>[2x]MDAQYDISFADVEKAHIN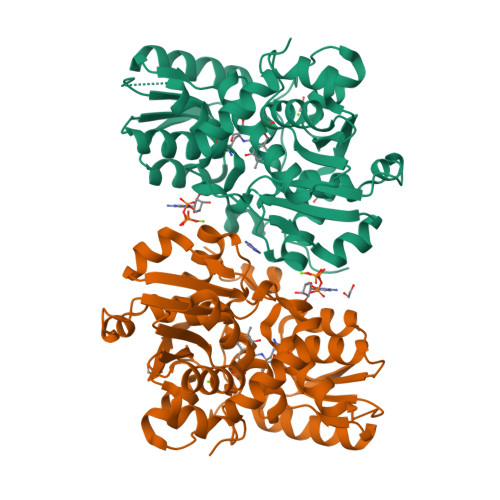IRDSIHLTPVLTSSILNQLTGRNLFFKCELFQKTGSFKIRGALNAVRSLVPDALERKPKAVVTHSSGNHGQALTYAAKLEGIPAYIVVPQTAPDCKKLAIQAYGASIVYCEPSDESRENVAKRVTEETEGIMVHPNQEPAVIAGQGTIALEVLNQVPLVDALVVPVGGGGMLAGIAITVKALKPSVKVYAAEPSNADDCYQSKLKGKLMPNLYPPETIADGVKSSIGLNTWPIIRDLVDDIFTVTEDEIKCATQLVWERMKLLIEPTAGVGVAAVLSQHFQTVSPEVKNICIVLSGGNVDLTSSITWVKQAERPASYQSVSVHHHHHHQ> MHHHHHHGMASM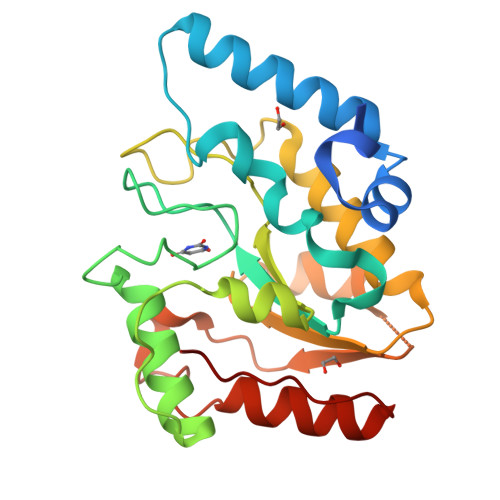TARPLSELVERGWAAALEPVADQVAHMGQFLRAEIAAGRRYLPAGSNVLRAFTFPFDNVRVLIVGQDPYPTPGHAVGLSFSVAPDVRPWPRSLANIFDEYTADLGYPLPSNGDLTPWAQRGVLLLNRVLTVRPSNPASHRGKGWEAVTECAIRALAARAAPLVAILWGRDASTLKPMLAAGNCVAIESPHPSPLSASRGFFGSRPFSRANELLVGMGAEPIDWRLP The covalent modification of target proteins with ubiquitin or ubiquitin-like modifiers is initiated by E1 activating enzymes, which typically transfer a single modifier onto cognate conjugating enzymes. UBA6 is an unusual E1 since it activates two highly distinct modifiers, ubiquitin and FAT10. In the presence of Mg-ATP, E1 catalyzes the acyl-adenylation of ubiquitin, initially forming a ubiquitin-AMP adduct. Subsequently, the E1 catalytic cysteine attacks the ubiquitin-AMP intermediate to form a thioester bond between the cysteine and the C-terminal glycine of ubiquitin, resulting in the formation of a covalent E1~ubiquitin adduct.

We initially determined the crystal structure of UBA6 in complex with ATP from an orthorhombic crystal form (space group P21221) at a resolution of 3.3 Å. Subsequently, crystals belonging to space group C2 became available, which diffracted anisotropically to 2.7/3.8 Å and, due to the higher resolution, will be described here. The cores of the two UBA6 molecules present in the asymmetric unit exhibit almost identical conformations with a root mean square deviation (rmsd) of 0.26 Å. However, the accessory components, the FCCH and SCCH domains as well as the UFD, display enhanced variability around this conserved core. The interactions between ATP and protein are completely conserved in the UBA6-ATP complex, thus illustrating the common framework for ATP-binding and hydrolysis in the E1 enzyme family. Due to the limited resolution of the UBA6-ATP complex the metal coordination cannot be fully resolved, however, a Mg2+-ion was modeled at the Mg(1) site, while a Ca2+-ion appears to be present in the Mg(2) site. In particular, the FCCH domain in UBA6 exhibits a movement of 7.5 Å away from the AAD-IAD core and hence away from where the ubiquitin molecule binds in the AAD domain as well as a 29° rotation. This change consequently introduces a broader cleft between the FCCH domain and the core of UBA6. At the same time, interactions between the FCCH and SCCH are formed. In the B-chain there are extensive contacts involving a hydrophobic core formed by F217, L232 and I287 of the FCCH domain and the aliphatic part of S737 as well as P738 of the SCCH domain and two ion pairs involving E249 (FCCH) and R740 (SCCH) as well as R248 (FCCH) and E876 (SCCH).

>[2x]MEGSEPVAAHQGEEASCSSWGTGSTNKNLPIMSTASVEIDDALYSRQRYVLGDTAMQKMAKSHVFLSGMGGLGLEIAKNLVLAGIKAVTIHDTEKCQAWDLGTNFFLSEDDVVNKRNRAEAVLKHIAELNPYVHVTSSSVPFNETTDLSFLDKYQCVVLTEMKLPLQKKINDFCRSQCPPIKFISADVHGIWSRLFCDFGDEFEVLDTTGEEPKEIFISNITQANPGIVTCLENHPHKLETGQFLTFREINGMTGLNGSIQQITVISPFSFSIGDTTELEPYLHGGIAVQVKTPKTVFFESLERQLKHPKCLIVDFSNPEAPLEIHTAMLALDQFQEKYSRKPNVGCQQDSEELLKLATSISETLEEKPDVNADIVHWLSWTAQGFLSPLAAAVGGVASQEVLKAVTGKFSPLCQWLYLEAADIVESLGKPECEEFLPRGDRYDALRACIGDTLCQKLQNLNIFLVGCGAIGCEMLKNFALLGVGTSKEKGMITVTDPDLIEKSNLNRQFLFRPHHIQKPKSYTAADATLKINSQIKIDAHLNKVCPTTETIYNDEFYTKQDVIITALDNVEARRYVDSRCLANLRPLLDSGTMGTKGHTEVIVPHLTESYNSHRDPPEEEIPFATLKSFPAAIEHTIQWARDKFESSFSHKPSLFNKFWQTYSSAEEVLQKIQSGHSLEGCFQVIKLLSRRPRNWSQCVELARLKFEKYFNHKALQLLHCFPLDIRLKDGSLFWQSPKRPPSPIKFDLNEPLHLSFLQNAAKLYATVYCIPFAEEDLSADALLNILSEVKIQEFKPSNKVVQTDETARKPDHVPISSEDERNAIFQLEKAILSNEATKSDLQMAVLSFEKDDDHNGHIDFITAASNLRAKMYSIEPADRFKTKRIAGKIIPAIATTTATVSGLVALEMIKVTGGYPFEAYKNCFLNLAIPIVVFTETTEVRKTKIRNGISFTIWDRWTVHGKEDFTLLDFINAVKEKYGIEPTMVVQGVKMLYVPVMPGHAKRLKLTMHKLVKPTTEKKYVDLTVSFAPDIDGDEDLPGPPVRYYFSHDTD> GGAGUUCACCGAGGCCACGCGG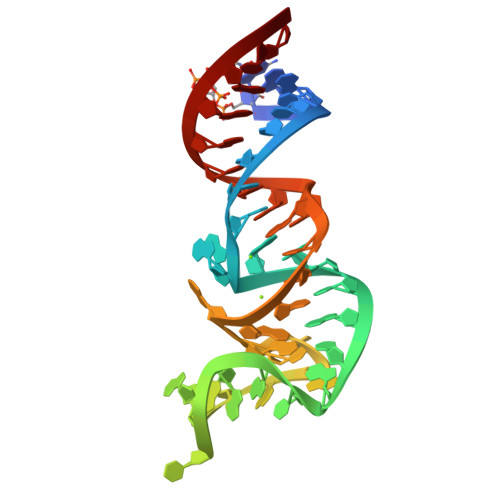AGUACGAUCGAGGGUACAGUGAAUU> ATQGVFTLPANTRFGVTAFANSSGTQTVNVLVNNETAATFSGQSTNNAVIGTQVLNSGSSGKVQVQVSVNGRPSDLVSAQVILTNEL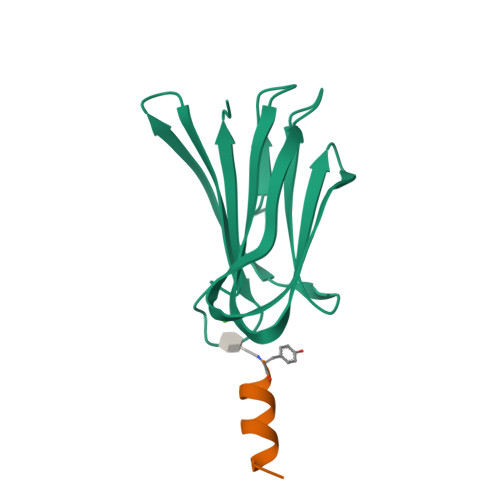NFALVGSEDGTDNDYNDAVVVINWPLG;> YKKALKKLAKLL>[2x]AKQKKEKVWAHYEEQPVEEVMPVLEEKERSASYKPVFVTEITDDLHFYVQDVETG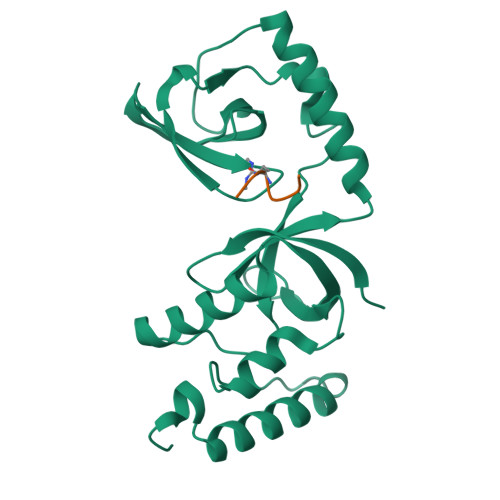TQLEKLMENMRNDIASHPPVEGSYAPRRGEFCIAKFVDGEWYRARVEKVESPAKIHVFYIDYGNREVLPSTRLGTLSPAFSTRVLPAQATEYAFAFIQVPQDDDARTDAVDSVVRDIQNTQCLLNVEHLSAGCPHVTLQFADSKGDVGLGLVKEGLVMVEVRKEKQFQKVITEYLNAQESAKSARLNLWRYGDFRADDADEFGYSR;>[2x]RGRARGQE> DTHWFHRNPLKATAPVSFNYYGVVTGPSASKICNDLRSSRARLLELFTDLSCNPEMMKNAAD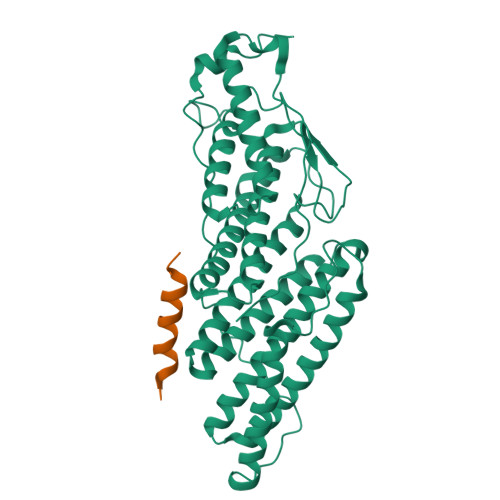SYFSLLQGFINSLDESTQESKLRYIQNFKWTDTLQGQVPSAQQDAVFELISMGFNVALWYTKYASRLAGKENITEDEAKEVHRSLKIAAGIFKHLKESHLPKLITPAEKGRDLESRLIEAYVIQCQAEAQEVTIARAIELKHAPGLIAALAYETANFYQKADHTLSSLEPAYSAKWRKYLHLKMCFYTAYAYCYHGETLLASDKCGEAIRSLQEAEKLYAKAEALCKEYGETKGPGPTVKPSGHLFFRKLGNLVKNTLEKCQRENGFIYFQKIPTEAPQLELKANYGLVEPIPFEFPPTSVQWTPETLAAFDLTKRPKDDSTKPKPEEEVKPVKEPDIKPQKDTGCYIS;> DNMDIDKVDELMQDIADQQELAEEISTAISKPVGFGEEFDEDELMAELEELEQEELDKNLLEISGPETVPLPNVPSIALPSKPAKKKEEEDDDMKELENWAGSM> LEDVVVQAPTQVPG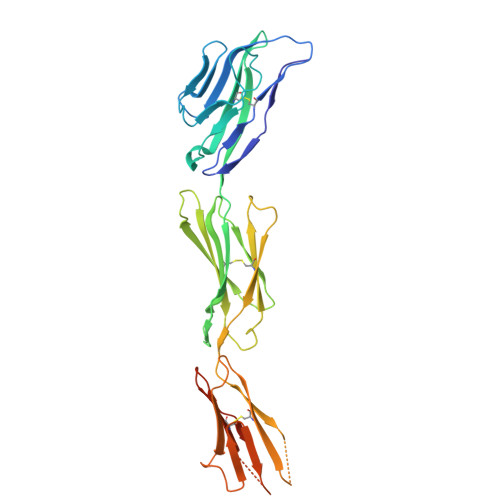FLGDSVTLPCYLQVPNMEVTHVSQLTWARHGESGSMAVFHQTQGPSYSESKRLEFVAARLGAELRNASLRMFGLRVEDEGNYTCLFVTFPQGSRSVDIWLRVLAKPQNTAEVQKVQLTGEPVPMARCVSTGGRPPAQITWHSDLGGMPNTSQVPGFLSGTVTVTSLWILVPSSQVDGKNVTCKVEHESFEKPQLLTVNLTVYYPPEVSISGYDNNWYLGQNEATLTCDARSNPEPTGYNWSTTMGPLPPFAVAQGAQLLIRPVDKPINTTLICNVTNALGARQAELTVQVKEGPPTSHHHHHH> MATPDQKSPNVLLQNLCCRILGKSEADVAQQFQYAVRVIGSNFAPTVERDEFLVAEKIKKELTRQRREADAALFSELHRKLHSQGVLKNKWSILYLLLSLSEDPRKQPSKVSGYAALFAQALPRDAHSTPYYYARPQSLPLNYQERGAPSAQSAGSAGSSGVSSLGTYALNGPTPPPPPPALLPGQPLPAPGVGDGLRQQLGSRLAWTLTASQPSLPSTTSKAVPSSGSRGAARPRREGDAAAGAVEVTEAALVRDI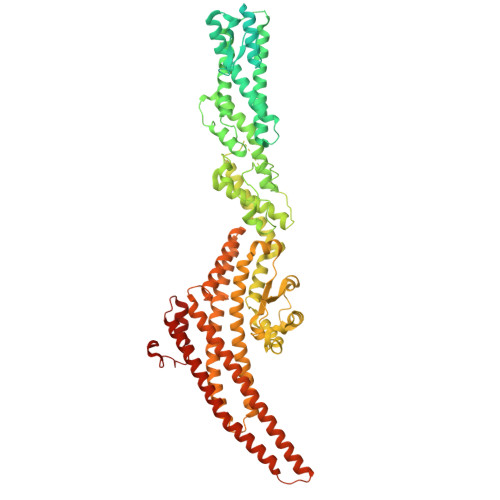LYVFQGIDGKHVKMSNADNCYTVEGKANLSKSLRDTAVRLAELGWLHNKIRKYTDQRSLDRSFGLVGQSFCAALHQELREYYRLLSVLHSQLQLEDDQGVNLGLESSLTLRRLLVWTYDPKMRLKTLAALVDHCQGRKGGELASAVHAYTKTGDPYARSLVQHILSLVSHPVLSFLYRWIYDGELEDTYHEFFVASDPAVKADRLWHDKYALRKPMIPSFMTMDQCRKVLLIGKSINFLHQVCHDQTPTTKMIAVTKSAESPQDAADLFTDLENAFQGKIDAAYFETSKYLLDVLNKKYSLLDHMQAMRRYLLLGQGDFIRHLMDLLKPELVRPATTLYQHNLTGILETAVRATNAQFDSPEILKRLDVRLLEVSPGDTGWDVFSLDYHVDGPIATVFTRECMSHYLRAFNFLWRAKRVEYILTDIRKGHMCNARLLRSMPEFSGVLHHCHILASEMVHFIHQMQYYVTFEVLECSWDELWNRVQRAQDLDHIIAAHEAFLGTVISRCLLDSDSRALLNQLRAVFDQIIELQNTQDAIYRAALEELQRRLQFEEKKKQREAEGQWGVSAAEEEQEKRRVQEFQESIPKMCSQLRILTHFYQGVVQQFLVSLTTSSDESLRFLSFRLDFNEHYRAREPRLRVSLGTRGRRSSHT> SVAHGFLITRHSQTTDAPQCPQGTLQVYEGFSLLYVQGNKRAHGQDLGTAGSCLRRFSTMPFMFCNINNVCNFASRNDYSYWLSTPEPMPMSMQPLKGQSIQPFISRCAVCEAPAVVIAVHSQTIQIPHCPQGWDSLWIGYSFMMHTSAGAEGSGQALASPGSCLEEFRSAPFIECHGRGTCNY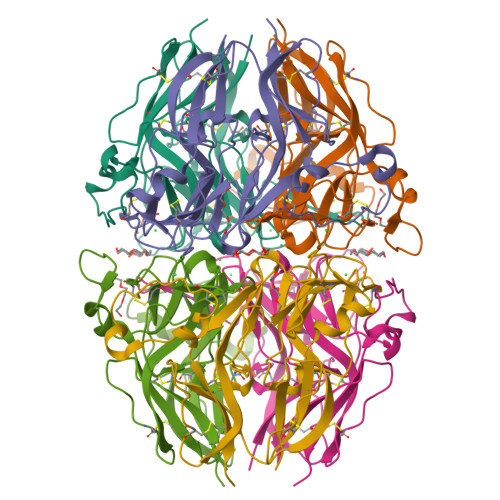YANSYSFWLATVDVSDMFSKPQSETLKAGDLRTRISRCQVCMKRT> VEGRFQLVAPYEPQGDQPQAIAKLVDGLRRGVKHQTLLGATGTGKTFTISNVIAQVNKPTLVIAHNKTLAGQLYSELKEFFPHNAVEYFVCYYDYYQPEAYVPQTDTYIEKDAKINDEIDKLRHSATSALFERRDVIIVASVSSIYGLGSPEEYRELVVSLRVGMEIERNALLRRLVDIQYDRNDIDFRRGTFRVRGDVVEIFPASRDEHSIRVEFFGDEIERIREVDALTGEVLGEREHVAIFPASHFVTREEKMRLAIQNIEQELEERLAELRAQGKLLEAQRLEQRTRYDLEMMREMGFSSGIENYSRHLALRPPGSTPYTLLDYFPDDFLIIVDESHVTLPQLRGMYNGDRARKQVLVDHGFRLPSALDNRPLTFEEFEQKINQIIYVSATPGPYELEHSPGVVEQIIRPTGLL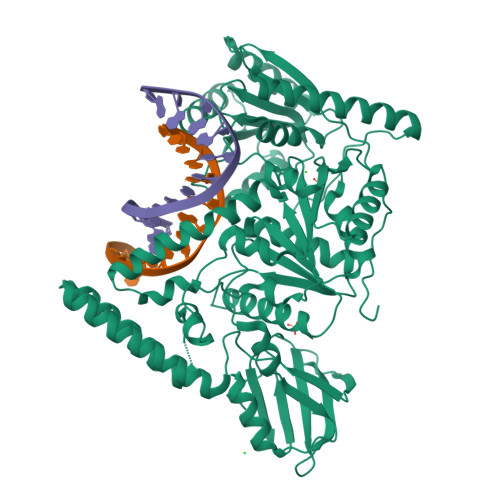DPTIDVRPTKGQIDDLIGEIRERVERNERTLVTTLTKKMAEDLTDYLKEAGIKVAYLHSEIKTLERIEIIRDLRLGKYDVLVGINLLREGLDIPEVSLVAILDADKEGALRSERSLIQTIGRAARNANGHVIMYADTITKSMEIAIQETKRRRAIQEEYNRKHGIVPRTVKKEIR5-bromo-1-(beta-D-glucopyranosyl)pyrimidine-2,4(1H,3H)-dione 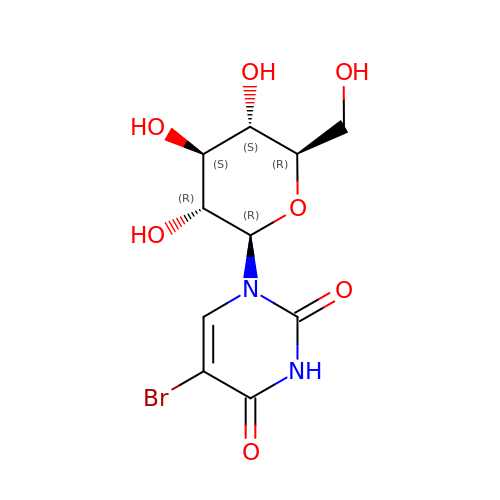| C10 H13 Br N2 O7 | QNNGZNNVDUDIOK-XSEHCYKFSA-N(2R)-3-(cyclohexylamino)-2-hydroxypropane-1-sulfonic 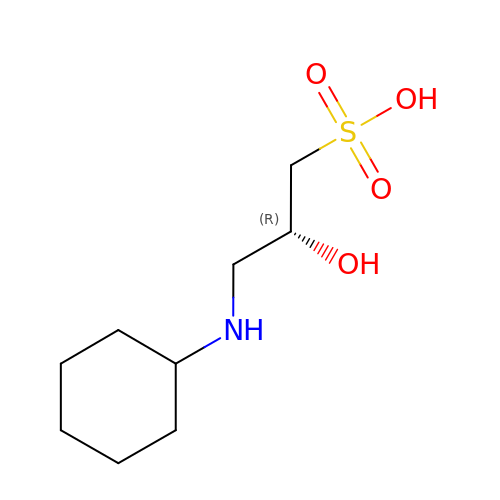acid | C9 H19 N O4 S | INEWUCPYEUEQTN-SECBINFHSA-N> METDLNSQDRKDLDKFIKFFALKTVQVIVQARLGEKICTRSSSSPTGSDWFNLAIKDIPEVTHEAKKALAGQLPAVGRSMCVEISLKTSEGDSMELEIWCLEMNEKCDKEIKVSYTVYNRLSLLLKSLLAITRVTPAYRLSRKQGHE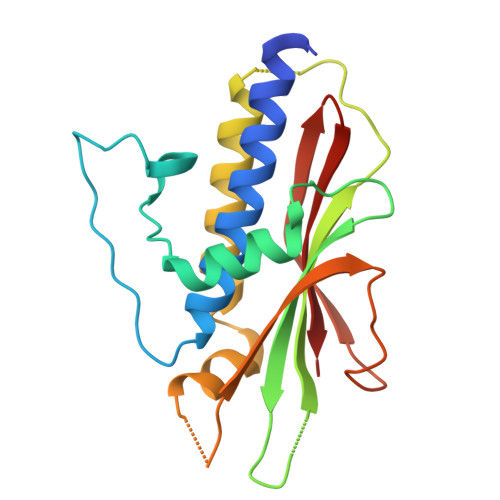YVILYRIYFGEVQLSGLGEGFQTVRVGTVGTPVGTITLSCAYR Aurora A is a serine/threonine protein kinase that plays an important role in controlling early stages of mitosis, including centrosome maturation and separation, mitotic entry, and bipolar spindle formation. Localization and enzymatic activity of Aurora A are regulated by its interaction with the spindle assembly factor TPX2. We have used fragment-based, structure-guided lead discovery to develop small molecule inhibitors of the Aurora A-TPX2 protein–protein interaction (PPI). The initial fragment hits identified from screening with the ATP site blocked by a high-affinity inhibitor were very weakly active, but guided by continuous crystallographic analysis of the inhibitors in complex with Aurora A, we were able to increase target affinity by more than 10,000-fold, clearly demonstrating the ability of fragment-based and structural biology approaches to develop potent PPI inhibitors when a suitable binding pocket is present. These compounds occupy a hydrophobic pocket on the surface of Aurora A, discrete from its ATP-binding catalytic site, which forms the interaction surface for a linear N-terminal segment of the interacting peptide from TPX2.

An early modification was to change the phenol group of 2 into indole while replacing the trifluoromethoxy with a smaller chlorine to give 3, which improved the KD to 1.26 μM. The indole-aryl core of the molecule lays in a hydrophobic pocket assembled from Leu169, Leu178, Val182, Val206, and the side chain of Lys166. The indole nitrogen proton forms a hydrogen bond with the side chain of Glu170 thus mimicking the phenol of Tyr8 of TPX2. The carboxylic acid group was observed to interact with Lys166 and His201. Furthermore, the electron density supported it being twisted from the plane of the indole ring in order to form a salt-bridge with Aurora A. Our analysis of ligands in PDB and CSD45 databases shows that carboxylic acids are more commonly in-plane with the aromatic ring (data not shown) and presumably this twisting incurs an energetic penalty upon binding.

> MGRQWALEDFEIGRPLGKGKFGNVYLAREKQSKFILALKVLFKAQLEKAGVEHQLRREVEIQSHLRHPNILRLYGYFHDATRVYLILEYAPLGTVYRELQKLSKFDEQRTATYITELANALSYCHSKRVIHRDIKPENLLLGSAGELKIADFGWSVHAPSSRRTTLAGTLDYLPPEMIEGRMHDEKVDLWSLGVLCYEFLVGKPPFEANTYQETYKRISRVEFTFPDFVTEGARDLISRLLKHNPSQRPMLREVLEHPWITANSS> GSHMEGAGAGSGFRKELVSRLLHLHFKDDKTKVSGDALQLMVELLKVFVVEAAVRGVRQAQAEDALRVDVDQLEKVLPQL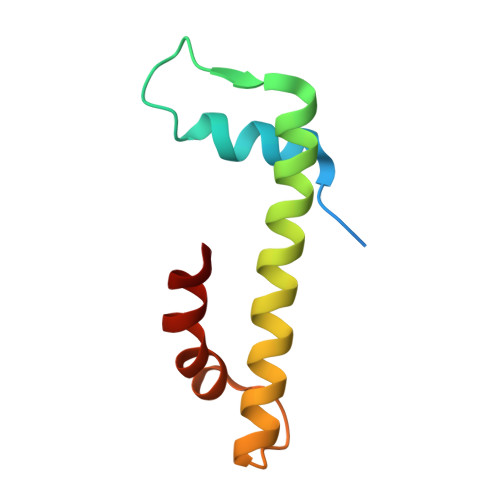LLDF In this process, small GTPase Rab5 functions as a master regulator of the early endosomal biogenesis. Rabex-5 is a specific GEF for Rab5, Rab17, and Rab21. Rabaptin-5 is a key effector of Rab5 and plays an important role in both homotypic and heterotypic fusions of early endosomes. The GEF activity of Rabex-5 is autoinhibited by its CC domain and is activated by the binding of Rabaptin-5 via its C2-1 domain.

In the Rabex-5CC structure, Rabex-5CC also forms a long α-helix (about 65 Å) and the four Rabex-5CC in the asymmetric unit form a tight four-helix bundle via the nonpolar surface. Rabex-5CC forms a stable amphipathic α-helix that tends to bury its nonpolar surface via oligomerization or interaction with the C-terminal regions of Rabaptin-5C212. The nonpolar surface of Rabex-5CC has good chemical and geometrical complementarities with the nonpolar surface groove of the GEF domain and thus might be able to bind there to block the substrate binding and hence autoinhibit the GEF activity as proposed by Delprato and Lambright (2007). Nonetheless, our structural and biochemical data show that although Rabex-5CC alone exists as a stable helix in both solution and crystal structure, it cannot form a stable complex with the GEF domain as shown by both GST pull-down assay and ITC analysis (data not shown).

>GSHMQMYKNLDLLSQLNERQERIMNEAKKLEKDLIDWTDGIAREVQDIVEK[4x]> ASLAADTPTACCFSYTSRQIPQNFIADYFETS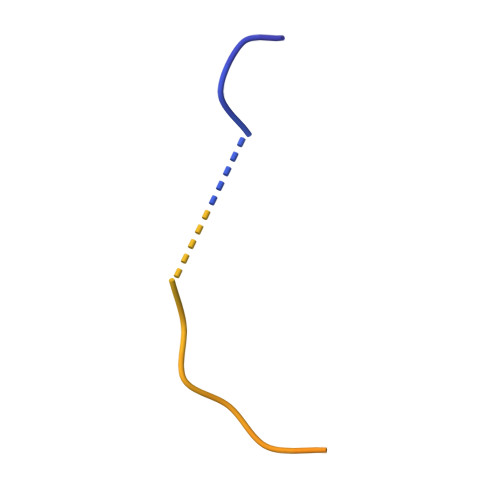SQCSKPGVIFLTKRSRQVCADPSEEWVQKYVSDLELSA> XEIAALKXENAAL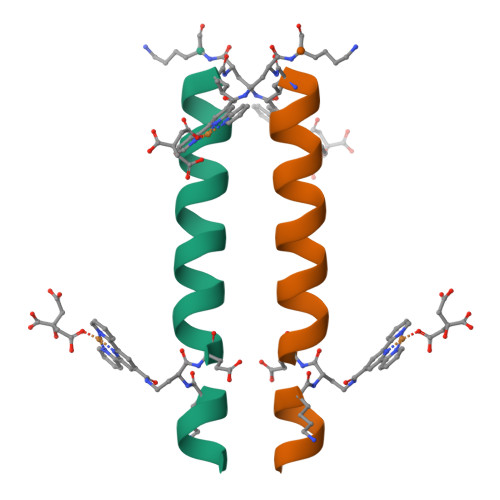KEEIAALKKEIAALXKGX> MLAEVLRDNGYHEYRARLQALLDIPELASDFEI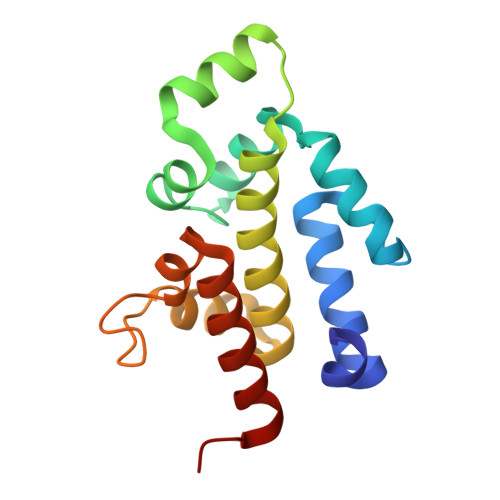HTRITDGFAATWLVKLTERGVLTPVERDQIIPLRTLKSRIERDQPLTVDESDRLFRSAHITAMAEAVFGEAGKAKRWLSKPKERFSGLTPMQMLTTQQGTTQVEEMLLQIAEGYGL>[2x]ASNFDCCLGYTDRILHPKFIVGFTRQLANEG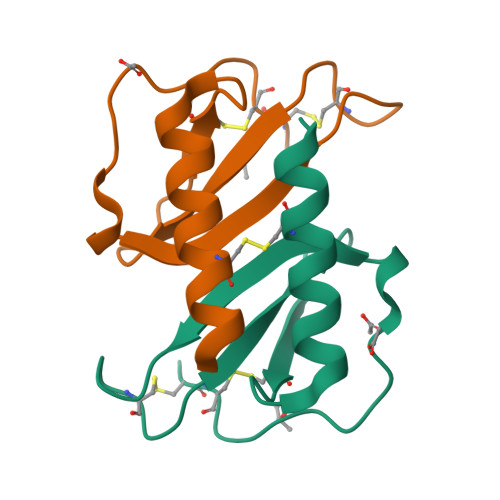CDINAIIFHTKKKLSVCANPKQTWVKYIVRLLCKKVKNM>[2x]WKEIKFEFDTIDPADSFSGASPERKAAVALRSLFTFVAARVVLEQLQGPGGPETTYNQQAYLDLMDFLGTPMKGDGGDEWMAAVMRKNHALALRLMEVREAYLDEFEWGKTMEMASRETREANTRLMRAAAM;> WKEIKF

Our data demonstrate that RbcX-II from the green algae C. reinhardtii functions as a bona fide Rubisco assembly chaperone, despite its considerable evolutionary distance from cyanobacterial and eukaryotic RbcX-I proteins. Like all other known RbcX proteins, CrRbcX-IIa is an arc-shaped dimer with a central hydrophobic cleft that binds the C-terminal sequence of the RbcL subunit. Conserved polar residues at the corners of RbcX make critical contacts to the N-domain of an adjacent RbcL, thereby stabilizing the RbcL anti-parallel dimer in a state competent for assembly to the RbcL8 core complex of Rubisco. The green algae Chlamydomonas reinhardtii contains two RbcX-II sequences (CrRbcX-IIa and CrRbcX-IIb, orthologs of AtRbcX-II) and no RbcX-I ortholog.

Taking advantage of the finding that the N-terminus of RbcX binds into the central cleft, we therefore generated a fusion construct between CrRbcX-IIa and the C-terminal recognition motif in CrRbcL. In this construct, residues 462–473 of CrRbcL (sequence WKEIKFEFDTID) are directly linked to residue Pro37 at the N-terminus of CrRbcX-IIa(37–156), with the new N-terminus of the fusion protein starting with Trp462 of the RbcL sequence. This fusion protein readily crystallized and the structure was solved at 1.97 Å resolution. Difference electron density along the hydrophobic cleft could be assigned to the RbcL residues 462–467 (WKEIKF). Residues 468–473 (EFDTID) of RbcL as well as residues 37–43 of CrRbcX-IIa were disordered. The sidechains of Ile465 and Phe467 point into hydrophobic pockets surrounded by Phe60/Arg64/Leu67/Leu92 and Leu57/Phe60/Met96, respectively. The sidechain of Lys463 points towards the C-terminal end of helix α2 and Asp90. The peptide is oriented more towards helix α2 in the cyanobacterial structure, whereas it assumes a deeper and more central position in the hydrophobic cleft of CrRbcX-IIa. Consistently, density for the bound peptide sequence is only discernible until the first Phe residue (Phe467) in the complex structure. The loop insertion between helices α1 and α2 of CrRbcX-IIa, which is ordered in the structure of the CrRbcL(462–474)-RbcX-IIa(37–156) fusion protein, would extend into a shallow groove of the RbcL dimer surface.>[2x]GHMPNIPPPFTAPYAPDDAEIAARLLPASHLSPPQEARIHRTATRLIEAIRKRDDRLGGVEDMLREFALSTKEGLALMVLAEALLRVPDARTADQFIEDKLGEGDFIHHETKSTAFLVNASAWALGLSARVIQPGETPDGTIGRLVKRLGAPAVRTATRQAMRLMGNHFVLGETIEQALERGKPRSGQKTRYSFDMLGEGARTAADARRYFDAYASAIETIGKAAGNHALPDRPGISVKLSALHPRFEAISRARVMVELVPQLLDLAQRAKAHDLNFTVDAEEADRLELSLDVIAATLADPSLKGWDGFGLAIQAYQKRASAVIDYVDALARAHDRKLMVRLVKGAYWDTEIKRAQERGLDGYPVFTRKAMTDLNYVACASKLLALRPRIFPQFATHNA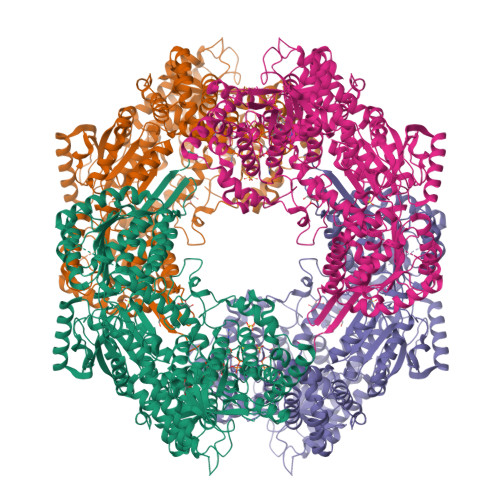LTVATVLEMAEGSSGFEFQRLHGMGEALYEQLAKDHADIAYRTYAPVGSHRDLLAYLVRRLLENGANSSFVAQAADYRVPVPALLQRPADAIVRPQAAAHPRIPLPCDLFAPERRNSRGVEFGARTALDQLLTDVKAETGDLKPIADATPDQAHAAVAAARAGFAGWSRTPAGIRAAALEQAAHLLESRSAHFIALLQREGGKTLDDALSELREAADFCRYYAAQGRKLFGSETAMPGPTGESNALTMRGRGVFVAISPWNFPLAIFLGQVTAALMAGNSVVAKPAEQTPRIAREAVALLHEAGIPKSALYLVTGDGRIGAALTAHPDIAGVVFTGSTEVARSINRALAAKDGPIVPLIAETGGINAMIADATALPEQVADWVVTSAFRSAGQRCSALRLLFVQEDVADRMIEMVAGAARELKIGDPSDVATHVGPVIDVEAKQRLDAHIARMKTEARLHFAGPAPEGCFVAPHIFELTEAGQLTEEVFGPILHVVRYRPENLERVLRAIERTGYGLTLGVHSRIDDSIEAIIDRVQVGNIYVNRNMIGAVVGVQPFGGNGLSGTGPKAGGPHYLARFATEQTVTINTAAAGGNAALLAGEE> SRLVEPYLDGYATSNVTTQIGTHAYLPCRVKQL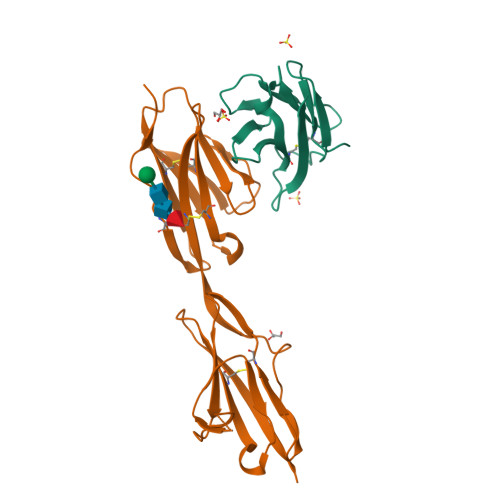GNKSVSWIRLRDGHILTVDRAVFIADQRFLAIKQPDKYWTLQIKYVQARDAGSYECQVSTEPKVSARVQLQVVVPHHHHHH;> SRLDPDPEFIGFINNVTYPAGREAILACSVRNLGKNKVGWLRASDQTVLALQGRVVTHNARISVMHQDMHTWKLKISKLRESDRGCYMCQINTSPMKKQVGCIDVQVPPDIINEESSADLAVQEGEDATLTCKATGNPQPRVTWRREDGEMILIRKPGSRELMKVESYNGSSLRLLRLERRQMGAYLCIASNDVPPAVSKRVSLSVHHHHHHH>MNTAVEPYKASSFDDTHKLTVEKHGHTALITINHPPANTWDRDSLIGLRQLIEHLNRDDDIYALVVTGQGPKFFSAGADLNMFADGDKARAREMARRFGEAFEALRDFRGVSIAAINGYAMGGGLECALACDIRIAERQAQMALPEAAVGLLPCAGGTQALPWLVGEGWAKRMILCNERVDAETALRIGLVEQVVDSGEARGAALLLAAKVARQSPVAIRTIKPLIQGARERAPNTWLPEERERFVDLFDAQDTREGVNAFLEKRDPKWRNCLEHHHHHH[6x]

In P. aeruginosa, the gene PA0745 encodes a putative crotonase, named dspI, which has been shown to be responsible for the CDA biosynthesis. The structural studies confirmed the catalytic features of DspI as an enoyl-coenzyme A (CoA) hydratase that catalyzes the dehydration of 3-hydroxydecanoyl-CoA during CDA synthesis. DspI is a α/β protein composed of six perpendicular antiparallel β-strands surrounded by eleven α-helices. It can be divided into two domains: the N-terminal spiral domain (α1–α8 and β1–β6) and the C-terminal trimerization domain (α9-end).

The proteins were crystallized in two different space groups. The P31 form has six molecules and the P6322 form has only one molecule per asymmetric units. The atomic coordinates from the two space groups were refined at a resolution of 2.10 Å and 2.25 Å. In both crystal forms, the first eight residues have not been modeled because of the poor density in this region. The C-terminal segment (residue 252–272) is further missing in the P6322 form. Thus, the structure of the P31 form is used for most of the descriptions in this study, unless otherwise specified. Hexamer organizations could be generated by applying the symmetry operations in both crystal forms. The hexamer is a dimer of two stacked trimers and each subunit possesses the canonical crotonase fold. In DspI, the C-terminal residue 252–272 (average B factor 73.54 Å2) is more flexible than the remainder of the trimerization domain (average B factor 41.71 Å2). It protrudes away from its own subunit and covers the neighboring monomer within the same trimer.> MASDYKDDDDKLHLILLPATGNVAENS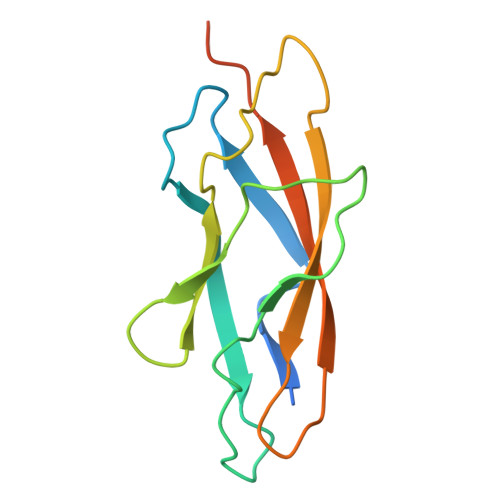PPGTSVHKFSVKLSASLSPVIPGFPQIVNSNPLTEAFRVNWLSGTYFEVVTTGMEQLDFETGPNIFDLQIYVKDEVGVTDLQVLTVQVTDVNEPPGGTKHHHHHH>MKVGIIMGSVRAKRVCPEIAAYVKRTIENSEELIDQKLKIQVVDL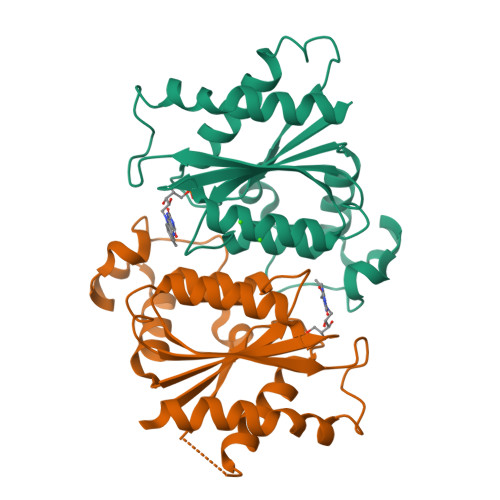QQIALPLYEDDDELIPAQIKSVDEYADSKTRSWSRIVNALDIIVFVTPQYNWGYPAALKNAIDRLYHEWHGKPALVVSYGGHGGSKCNDQLQEVLHGLKMNVIGGVAVKIPVGTIPLPEDIVPQLSVHNEEILQLLASCIETTRNK[2x]>GMMNETLKVIAERYSCRDFKNEMPSDELLQAIAEAAIQAPSGMNRQAWRVIVVKNKELMQEMEAEGLAYLAGMEDQSSYNRIMERGGRLFYGAPCMIVVPIDPTQYGPALVDCGILCQTIALAATSLGIANIMCGYTGL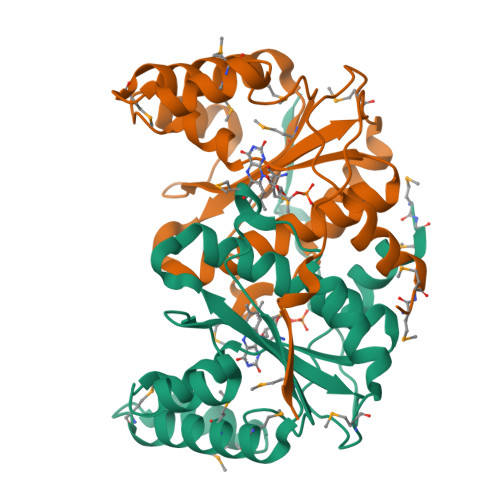AFASGLRAEEFSKRLGFPEGYAFGCSVLLGHANTTKPPHVPDKDKITYVE[4x]> GPLGSHMSQAVQTNGTQPLSKTWELSLYELQRTPQEAITDGLEIVVSPRSLHSELMCPICLDMLKN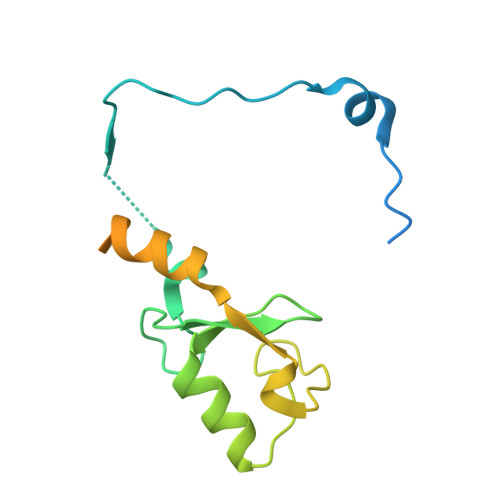TMTTKECLHRFCADCIITALRSGNKECPTCRKKLVSKRSLRPDPNFDALISKIYPSRDEYEAHQERVLARINKHNNQQALSHSIEEGLKIQAMNRLQRG> SQAEVLHLCRSLEVGTVMTLFYSKKSQRPERKTFQVKLETRQITWSRGADKIEGSIDIREIKEIRPGKTSRDFDRYQEDPAFRPDQSHCFVILYGMEFRLKTLSLQATSEDEVNMWIKGLTWLMEDTLQAATPLQIERWLRKQFYSVDRNREDRISAKDLKNMLSQVNYRVPNMRFLRERLTDLEQRSGDITYGQFAQLYRSLMYSAQKTMDLPFLETNTLRTGERPELCQVSLSEFQQFLLEYQGELWAVDRLQVQEFMLSFLRDPLREIEEPYFFLDELVTFLFSKENSVWNSQLDAVCPETMNNPLSHYWISSSHNTYLTGDQFSSESSLEAYARCLRMGCRCIELDCWDGPDGMPVIYHGHTLTTKIKFSDVLHTIKEHAFVASEYPVILSIEDHCSIAQQRNMAQHFRKVLGDTLLTKPVDIAADGLPSPNQLKRKILIKHKKLAEGSAYEEVPTSVMYSENDISNSIKNGILYLEDPVNHEWYPHYFVLTSSKIYYSEETSSDQGNEDEEEPKEASGSTELHSSEKWFHGKLGAGRDGRHIAERLLTEYCIETGAPDGSFLVRESETFVGDYTLSFWRNGKVQHCRIHSRQDAGTPKFFLTDNLVFDSLYDLITHYQQVPLRCNEFEMRLSEPVPQTN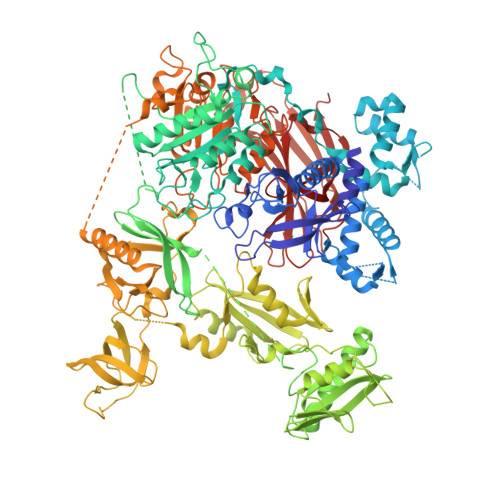AHESKEWYHASLTRAQAEHMLMRVPRDGAFLVRKRNEPNSYAISFRAEGKIKHCRVQQEGQTVMLGNSEFDSLVDLISYYEKHPLYRKMKLRYPINEEALEKIGSGSTFKCAVKALFDYKAQREDELTFTKSAIIQNVEKQDGGWWRGDYGGKKQLWFPSNYVEEMINPAILEPEREHLDENSPLGDLLRGVLDVPACQIAIRPEGKNNRLFVFSISMPSVAQWSLDVAADSQEELQDWVKKIREVAQTADARLTEGKMMERRKKIALELSELVVYCRPVPFDEEKIGTERACYRDMSSFPETKAEKYVNKAKGKKFLQYNRLQLSRIYPKGQRLDSSNYDPLPMWICGSQLVALNFQTPDKPMQMNQALFMAGGHCGYVLQPSTMRDEAFDPFDKSSLRGLEPCVICIEVLGARHLPKNGRGIVCPFVEIEVAGAEYDSTKQKTEFVVDNGLNPVWPAKPFHFQISNPEFAFLRFVVYEEDMFSDQNFLAQATFPVKGLKTGYRAVPLKNNYSEDLELASLLIKIDIFPAK N-[(E)-3-[(2R,3S,4R,5R)-3,4-dihydroxy-5-purin-9-yl-oxolan-2-yl]prop-2-enyl]-2,3-dihydroxy-5-nitro-benzamide 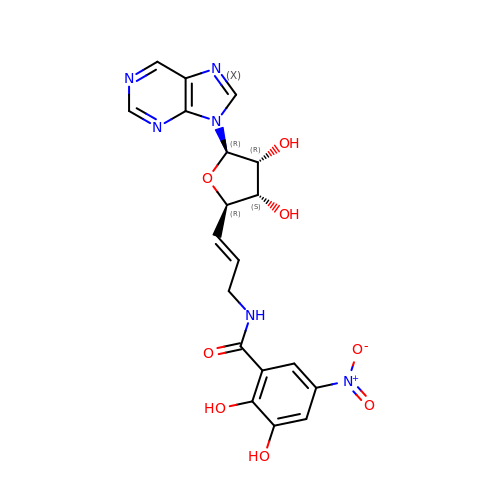| C19 H18 N6 O8 | CNQHTUXYFHTEGE-QFIYFXBNSA-N> M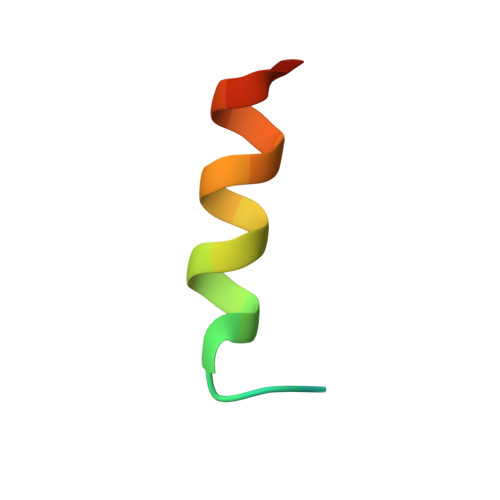QMNRYDQAATLRAKMEKRERVL> DIAVKSAASV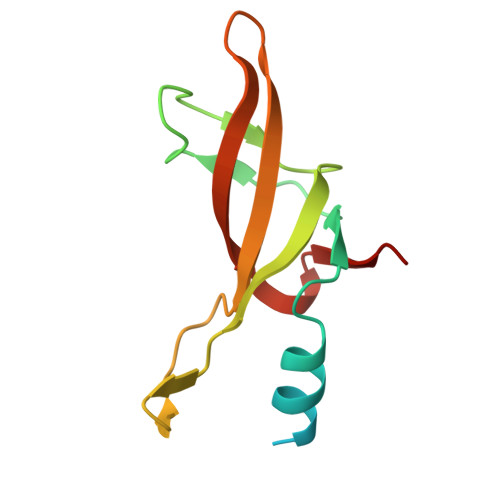DADADLSSSTSLETEEDEKAKEKIGARVRVTVPLKVYHVVRVPEVELMGMEGFIKDYVVLWKGKKISANLPFKVQFVKEIEGRGPVKFFTHLKEDEFELIDP>[6x]MHEPMKTLKNIHAEIRICQKFPKSTVQKRFSEFEELIKAASKNARNWKPISSVELFQGDSSLNELFEKLVIGTCELRDGELFENVNDLTINPSNIHVYKLHKDGPLSQNIGDDDGDESIIGSQLWQLPCVEFDSIWENLIYDSNLKNEVMSYVAALARLSEKHVNTKIINVNRLILLTGPPGTGKTSLCKGLAQHLSIRMNDKYSKSVMLEINSHSLFSKWFSESGKLVQKMFDQIDELAEDEKCMVFVLIDEVESLGMCRESSSSRSEPSDAIRAVNALLTQIDRIRRRDNVLILCTSNLESTLDKALVDRADIVKNVGQPSDFARYSMLKSSIMELARIGVVIDNEVHTDYWPQDICDTKAPRNEFTEILFKIAQEARGLSGRAISMLPTLVYSKSPEETITLPNCMNLFLEAVKERLSRNN

Here, we show that Pch2/TRIP13 comprises a new family of AAA+ ATPase protein remodelers, with a substrate-recognition domain similar to the NSF/p97/PEX1 remodeler family and a physical mechanism closely related to the bacterial ClpX unfoldase. Pch2/TRIP13 proteins are members of the functionally diverse AAA+ ATPase family. These proteins share a common architecture, with a family-specific N-terminal domain (NTD) responsible for localization or substrate recognition, and one or two AAA+ ATPase modules that typically assemble into a hexameric ring. We show that TRIP13 converts closed, active MAD2 to its inactive open conformer, and that p31(comet) functions as an adapter to recognize closed MAD2 and deliver it to TRIP13. Thus, TRIP13 regulates the SAC through MAD2 conformational conversion and safety belt disengagement, and a similar mechanism for HORMAD complex disassembly likely underlies the enzyme's regulatory functions in meiosis.

We attempted crystallization both in the presence and absence of nucleotides, and successfully determined the crystal structure of PCH-2 without added nucleotide to a resolution of 2.3 Å. While the PCH-2 NTD (residues 1–99 of 424) lacks detectable sequence homology to other proteins, the structure of this domain shows a clear relationship to the N-terminal substrate recognition domains of a AAA+ ‘classic remodeler’ sub-family that includes NSF, p97, and PEX1. In PCH-2, the NTD contains a single folded domain similar to the NSF/p97/PEX1 N-C subdomain, and as such does not share these proteins' substrate-binding hydrophobic cleft. As in other AAA+ ATPases, the PCH-2 hexamer assembles through interactions between each subunit's large AAA domain and the small AAA domain of a neighboring subunit, with the ATP-binding sites situated near the subunit interfaces. Although no nucleotides were added during purification or crystallization of PCH-2, we observed that two subunits in the hexamer (chains B and E) are bound to ADP, enabling a close analysis of PCH-2 active site structure. Pch2/TRIP13 proteins, in contrast, possesses only a single arginine finger (R312 in C. elegans PCH-2), and our PCH-2 structure shows that a conserved arginine (R385) is properly positioned to act as a Sensor-2 motif. Within the hexamer, four PCH-2 subunits adopt a ‘closed’ conformation equivalent to that observed in most AAA+ ‘classic remodeler’ structures, with the large and small AAA domains tightly associated around the ATP-binding site. Asymmetry in the PCH-2 hexamer arises from large conformational differences in the remaining two subunits (chains C and F, also bound to SO4−), situated on opposite ends of the extended hexamer. Instead, the PCH-2 structure closely resembles several prior structures of the ClpX unfoldase, which contain four ‘closed’ and two ‘open’ subunits arranged in the same pattern as in PCH-2.>[2x]MAHHHHHHESETTTSLVLERSLNRVHLLGRVGQDPVLRQVEGKNPVTIFSLATNEMWRSGDSEVYQLGDVSQKTTWHRISVFRPGLRDVAYQYVKKGSRIYLEGKIDYGEYMDKNNVRRQATTIIADNIIFLSDQTKEKELE;> SSSS

SSBP1 is a key protein for the mtDNA replication machinery. SSBP1 is required to stabilize single-stranded mtDNA (ssmtDNA) and stimulate DNA synthesis by POLG. SSBP1 encodes a mitochondrial ssDNA-binding protein and interacts with POLG and TWINKLE at the mitochondrial replication fork to stimulate the synthesis of mtDNA. During replication, SSBP1 binds to ssmtDNA as a tetramer and prevents reannealing and nucleolytic attacks.

However, these structures show different sequence assignments for the 15 amino acids at the C terminus. To clarify this issue, we solved the crystal structure of SSBP1 at a higher resolution and calculated the electron density maps. Arg38 is close to the surface that (in the homologues) binds the DNA. Importantly, the guanidinium nitrogens at the end of the Arg38 side chain interact with the side-chain Glu27 carboxylate group from molB. Thus, Arg38 participates in intermolecular contacts within the dimer (the same contact occurs between Arg38 molB and Glu27 molA). Arg107 is packed against a hydrophobic pocket at the dimer interface, where it interacts with main-chain carbonyls of both molB Arg28 (intradimer contact) and molB′ Phe139 (interdimer contact). Therefore, both arginines participate in AB (and BA) dimer interactions, whereas Arg107 additionally contacts the other dimer within the tetramer. Our molecular modeling on our new, higher resolution crystal structure of SSBP1 suggests that R38Q and R107Q substitutions may affect both multimerization of SSBP1 and DNA binding. The mutated Arg38Gln shorter side chain is unable to reach this region.Malonyl-coenzyme A decarboxylase (MCD) is found from bacteria to humans, has important roles in regulating fatty acid metabolism and food intake, and is an attractive target for drug discovery. The MCD monomer contains an N-terminal helical domain involved in oligomerization and a C-terminal catalytic domain. Unexpectedly, the MCD catalytic domain is structurally homologous to those of the GCN5-related N-acetyltransferase superfamily, especially the curacin A polyketide synthase catalytic module, with a conserved His-Ser/Thr dyad important for catalysis. The catalytic domain of MCD contains a central eight-stranded, mostly antiparallel β sheet (β1–β8) that is surrounded by at least 11 α helices (α1–α11).

After significant efforts at optimization and diffraction screening, we collected X-ray diffraction data for RpMCD, Agrobacterium vitis MCD (AvMCD), and Cupriavidus metallidurans MCD (CmMCD) at up to 2.3 Å resolution. We solved the structure of RpMCD by the selenomethionyl single-wavelength anomalous diffraction method and the structures of AvMCD and CmMCD by molecular replacement. RpMCD and AvMCD are also tetramers in solution, based on multiangle static light scattering studies (data not shown). Like HsMCD, the RpMCD and AvMCD tetramers are also dimer of dimers. However, the relative orientations of the dimers are substantially different. There is an insert of three additional helices (α5–α7) between strands β5 and β6 in HsMCD, RpMCD, and AvMCD, while CmMCD has an insert of five helices here.

> MAGTSFLSDLLSGVTERGRALLFSGSKARDRVVDTDIETLCEMLLSSRGEASGMAIAAEILDRWSRFNAAEAVQFLHMLSDRFGAEAAALDKAIDAYRTDKSPMAVIALHNAAEPRRQELLRRLNLAPNGTQKLVRMRERLLETKEDRADLGAVDTDFAHLFSSWFNRGFLTLQPIDWTTPAHILEKIIKYEAVHEIAGWEELRRRLAPADRRCFAFFHPRLRDDPLVFVEVALTRSIPSAIADVLDESRDHIGADTATTAVFYSISNCQDGLRGISFGNFLIKQVVEDLRRDLPGLKEFVTLSPVPGFARWISKIRDPKSGFPLSPEDRNTLVLLDDPTWPEDKARADAVERILLPLAARYFITERTPDNRPVDPVARFHLGNGARLERLNFLGDRSVKAMRQAHGLMVNYLYKLEDIETNHEALAQRGEVAASPAVKALQGKIEPILEHHHHHH The Eph receptors are the largest receptor tyrosine kinase family, and together with their cell surface-anchored ephrin ligands represent an important cell-cell communication system that regulates a multitude of physiological and pathological processes. The intracellular portion of the Eph receptors includes a juxtamembrane segment, the tyrosine kinase domain, a linker, a sterile alpha motif (SAM) domain, and a short C-terminal tail containing a PDZ domain-binding motif. EphA2 promotes cancer malignancy through a poorly understood non-canonical form of signaling involving serine/threonine phosphorylation of the linker connecting its kinase and SAM domains. The kinase-SAM linker contains a cluster of five serine/threonine residues that besides S897 include S892, T898, S899 and S901.

To determine whether the negative charges introduced by phosphorylation of the linker might affect the kinase-SAM domain arrangement, we solved the structures of two EphA2 phosphomimetic mutants. In the first, we replaced both S897 and S901 with glutamic acid, since glutamate is known to at least in part functionally mimic a phosphorylated residue when the effects of phosphorylation are due to the negative charge of phosphate. The structure of the EphA2 S897E/S901E double mutant shows a different kinase-SAM domain arrangement than EphA2 WT. In the single molecule of the structure, the SAM domain is completely detached from the kinase domain and the C-terminal part of the linker is fully extended. Unlike the EphA2 WT structure, the activation loop is fully resolved in the S897E/S901E mutant structure, potentially due to stabilizing crystal contacts. In the S897E/S901E structure, however, the central portion of the kinase-SAM linker adopts a conformation different from WT and appears to be stabilized by a salt bridge between E897 (replacing S897) and R890. Additionally, a key difference is evident in the αFG loop of the kinase domain, including W819 and adjacent residues, a region previously identified in EphA3 as part of an allosteric network connecting the juxtamembrane segment, activation loop and kinase-SAM linker. We did not observe any substantial differences in the overall fold of the individual domains between the WT and S897E/S901E structures, and all EphA2 molecules in both structures adopt the active DFG-in conformation. Supporting this hypothesis, E820 is in a different conformation in the EphA2 WT structure compared to the EphA2 S897E/S901E structure. The EphA2 5E envelope best fits the more elongated conformation of the EphA2 S897E/S901E crystal structure, but in general shows less agreement with the crystal structures, suggesting that the EphA2 intracellular region adopts an ensemble of conformations in solution that is shifted towards more elongated conformations by phosphomimetic negative charges in the linker.

> GPGDPHTYEDPNQAVLKFTTEIHPSCVTRQKVIGAGEFGEVYKGMLKTSSGKKEVPVAIKTLKAGYTEKQRVDFLGEAGIMGQFSHHNIIRLEGVISKYKPMMIITEYMENGALDKFLREKDGEFSVLQLVGMLRGIAAGMKYLANMNYVHRDLAARNILVNSNLVCKVSDFGLSRVLEDDPEATYTTSGGKIPIRWTAPEAISYRKFTSASDVWSFGIVMWEVMTYGERPYWELSNHEVMKAINDGFRLPTPMDCPSAIYQLMMQCWQQERARRPKFADIVSILDKLIRAPDSLKTLADFDPRVSIRLPETSGEEGVPFRTVSEWLESIKMQQYTEHFMAAGYTAIEKVVQMTNDDIKRIGVRLPGHQKRIAYSLLGLKDQVNTVGIPI> MAGERFPADFVWGAATAAYQIEGAVREDGRGVSIWDTFSHTPGKIADGTTGDVACDSYHRYGEDIGLLNALGMNAYRFSIAWPRIVPLGAGPINQAGLDHYSRMVDALLGAGLQPFVTLYHWDLPQPLEDRLGWGSRATATVFAEYADIVVRQLGDRVTHWATLNEPWCSAMLGYYLGVHAPGHTDLKRGLEASHNLLLGHGLAVQAMRAAAPQPLQIGIVLGLTPTYPASDSPEDVAAARRFDGFVNRWFLDPLAGRGYPQDMLDYYGAAAPQANPEDLTQIAAPLDWL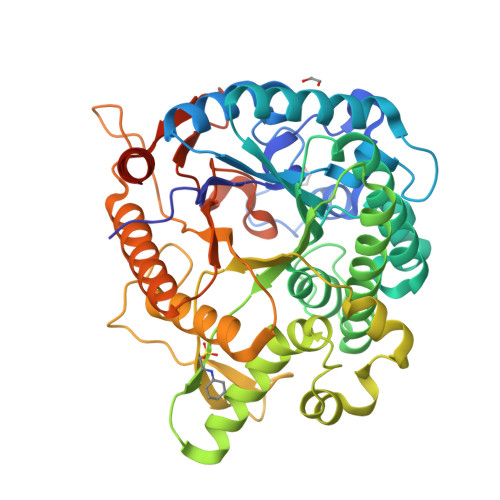GVNYYERMRAVDAPDASLPQAQRLDDPDLPHTADREVYPEGLYDILLRLHNDYPFRPLYITENGCALHDEIAEDGGIHDGQRQAFFEAHLAQLQRALAAGVPLKGYFAWSLLDNFEWAMGLSMRYGICYTNFETLERRIKDSGYWLRDFIAGQRGKLAALEHHHHHH2-(4-(2-methoxy-4-morpholinophenylamino)-1,3,5-triazin-2-ylamino)-N-methylbenzamide 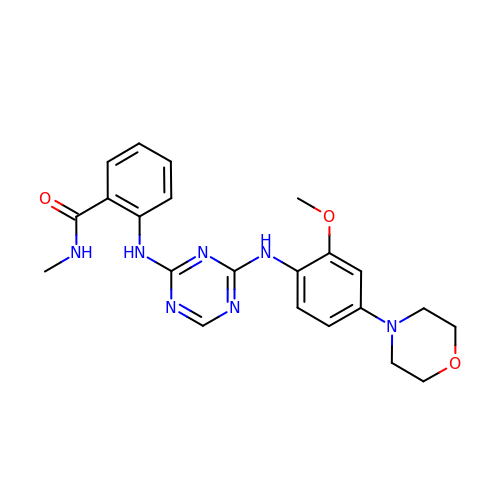| C22 H25 N7 O3 | MMFUMGAALISETK-UHFFFAOYSA-N>[8x]MKTSDANETEDHLESLICKVGEKSACSLESNLEGLAGVLEADLPNYKSKILRLLCTVARLLPEKLTIYTTLVGLLNARNYNFGGEFVEAMIRQLKESLKANNYNEAVYLVRFLSDLVNCHVIAAPSMVAMFENFVSVTQEEDVPQVRRDWYVYAFLSSLPWVGKELYEKKDAEMDRIFANTESYLKRRQKTHVPMLQVWTADKPHPQEEYLDCLWAQIQKLKKDRWQERHILRPYLAFDSILCEALQHNLPPFTPPPHTEDSVYPMPRVIFRMFDYTDDPEGPVMPGSHSVERFVIEENLHCIIKSHWKERKTCAAQLVSYPGKNKIPLNYHIVEVIFAELFQLPAPPHIDVMYTTLLIELCKLQPGSLPQVLAQATEMLYMRLDTMNTTCVDRFINWFSHHLSNFQFRWSWEDWSDCLSQDPESPKPKFVREVLEKCMRLSYHQRILDIVPPTFSALCPVNPTCIYKYGDESSNSLPGHSVALCLAVAFKSKATNDEIFSILKDVPNPNQDDDDDEGFSFNPLKIEVFVQTLLHLAAKSFSHSFSALAKFHEVFKTLAESDEGKLHVLRVMFEVWRNHPQMIAVLVDKMIRTQIVDCAAVANWIFSSELSRDFTRLFVWEILHSTIRKMNKHVLKIQKELEEAKEKLARQHKRRSDDDDRSSDRKDGVLEEQIERLQEKVESAQSEQKNLFLVIFQRFIMILTEHLVRCETDGTSVLTPWYKNCIERLQQIFLQHHQIIQQYMVTLENLLFTAELDPHILAVFQQFCALQA;>[8x]GAMSGGLLKALRSDSYVELSQYRDQHFRGDNEEQEKLLKKSCTLYVGNLSFYTTEEQIYELFSKSGDIKKIIMGLDKMKKTACGFCFVEYYSRADAENAMRYINGTRLDDRIIRTDWDAGFKEGRQYGRGRSGGQVRDEYRQDYDAGRGGYGKLAQNQ;>GAMGRGNYDAFRGQGGYPGKPRNRMVRGDPRAIVEYRDLDAPDDVDFF[8x]

The nuclear cap-binding complex (CBC) binds tightly to the 5′-cap structure (m7GpppN, where N is the first transcribed nucleotide) which is co-transcriptionally added to all nascent Pol II transcripts 25–50 nucleotides after initiation. CBC bound to capped RNA not only protects the transcript from decapping and subsequent further 5′-3′ degradation, but also acts as a platform for interaction with nuclear factors that determine the fate of the transcript. Here we take a biochemical and structural approach to investigate which binary and ternary complexes CBC can form with three nuclear factors, PHAX, ARS2 (arsenate resistance protein 2), and NELF (negative elongation factor), all of which directly interact with CBC and are involved in CBC-mediated transcript processing. We also determine crystal structures of CBC bound to ARS2 or NELF-E peptide that explain why CBC–ARS2–PHAX and CBC–NELF–E form mutually exclusive complexes.

Therefore to obtain a structure of the CBC–ARS2 complex, we co-crystallised m7GTP-CBC (CBP20-CBP80ΔNLS) with ARS2827–871. A P1 crystal form diffracting to 2.8 Å resolution showed convincing ARS2 peptide density. There are eight complexes in the asymmetric unit with variable occupancy of the ARS2 peptide, probably due to the relatively low affinity. The C-terminus of ARS2, which is only visible beyond residue 851, forms an extended chain that wraps around the CBP80–CBP20 interface, interacting with both subunits. The principle interacting regions of CBP80 are 460–463, 557–570, 607–616, and 647–651, and of CBP20 are 48–55 (β1–α2 loop of the RRM domain) and 71–80 (β2–β3 loop). There are two main interacting regions of the ARS2 peptide, residues 852-DPRAIVEYRD-861, notably Asp852, Arg854, and Tyr859, which bind in the “proximal” site and the extreme C-terminal residues 868-VDFF-871, notably Phe871, which bind in the “distal” site. The electron density is absent for the intervening residues 862-LDAPDD-867. In the proximal site, Asp852 electrostatically stabilises Arg854, whose guanidinium group stacks on Tyr461 of CBP80 and forms a salt bridge with Asp107 from CBP20 (left). In the distal site, the side chain of Phe871, the extreme C-terminal ARS2 residue, is buried in a hydrophobic pocket formed by CBP80 Ile609, Cys616, Met648, and His651 at the base of the long, solvent protruding coiled-coil of CBP80 (residues 650–705) (right). ITC measurements showed that the R854A/Y859A double mutation severely weakened the interaction with CBC, whereas F871D alone did not have a major effect.>MKKQTQLLSALALSVGLTLSASFQAVASIPGQVADQAPLPSLAPMLEKVLPAVVSVRVEGTASQGQKIPEEFKKFFGDDLPDQPAQPFEGLGSGVIINASKGYVLTNNHVINQAQKISIQLNDGREFDAKLIGSDDQSDIALLQIQNPSKLTQIAIADSDKLRVGDFAVAVGNPFGLGQTATSGIVSALGRSGLNLEGLENFIQTDASINRGNAGGALLNLNGELIGINTAILAPGGGSVGIGFAIPSNMARTLAQQLIDFGEIKRGLLGIKGTEMSADIAKAFNLDVQRGAFVSEVLPGSGSAKAGVKAGDIITSLNGKPLNSFAELRSRIATTEPGTKVKLGLLRNGKPLEVEVTLDTSTSSSASAEMITPALEGATLSDGQLKDGGKGIKIDEVVKGSPAAQAGLQKDDV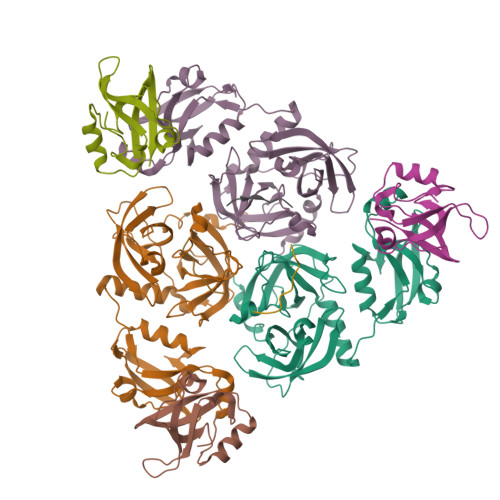IIGVNRDRVNSIAEMRKVLAAKPAIIALQIVRGNESIYLLMRLWHHHHHH[6x]> GKDDDNVETGAFDPSKPVAISDFTPKEGGAYQKLLIYGENFGTDVSKVKVKIGGKDAIVINVKSTYVYCFVPSGAFSGEIEITVGEGENAVTTTASTTFSYEKKMVVGTLCGYRNNRDDQGWRDGPFDGPEGVKCCGFSDNGRLAFDPLNKDHLYICYDGHKAIQLIDLKNRMLSSPLNINTIPTNRIRSIAFNKKIEGYADEAEYMIVAIDYDGKGDESPS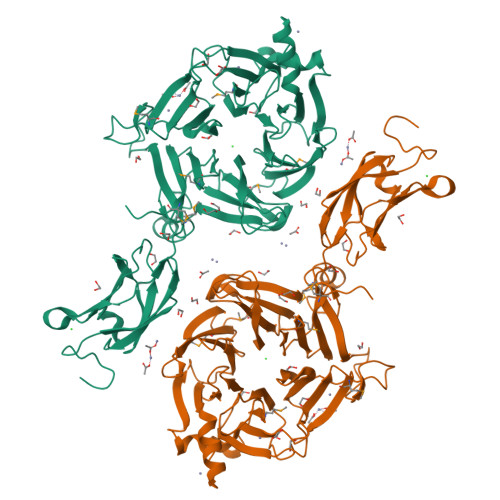VYIIKRNADGTFDDRSDIQLIAAYKQCNGATIHPINGELYFNSYEKGQVFRLDLVDYFKTIKNGGSWDPIVKNNPNTFKQLFTIADPSWEFQIFIHPTGKYAYFGVINNHYFMRSDYDEIKKEFITPYNFVGGYKQSGYRDDVGTEARMNNPCQGVFVKNPDYTGEEEYDFYFVDRLNFCVRKVTPEGIVSTYAGRGASTSLADGNQWGTDDGDLREVARFRDVSGLVYDDVKEMFYVHDQVGHTIRTISMEQEENVAGDENIPEDESTVESNE(2~{S})-2-azanyl-3-[4-[(2-nitrophenyl)methoxy]phenyl]propanoic 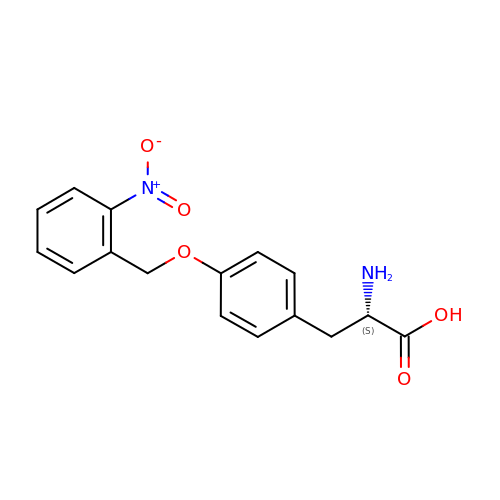acid | C16 H16 N2 O5 | NLFOHNAFILVHGM-AWEZNQCLSA-N5-nitro-1,2-benzoxazole | 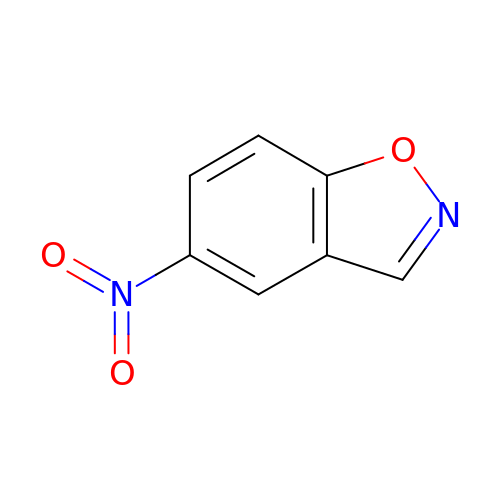C7 H4 N2 O3 | TWOYWCWKYDYTIP-UHFFFAOYSA-N>[2x]MAAQGPSPIPTNRLKQIAADACNDAIGSAEFYDHAKTEQWNHQIINTILKAVIAESQPSDSTTPPQFKFAVNSTIVQHLVPSSKLNKPAGGADDKPASTATSTDGKPHVGRRG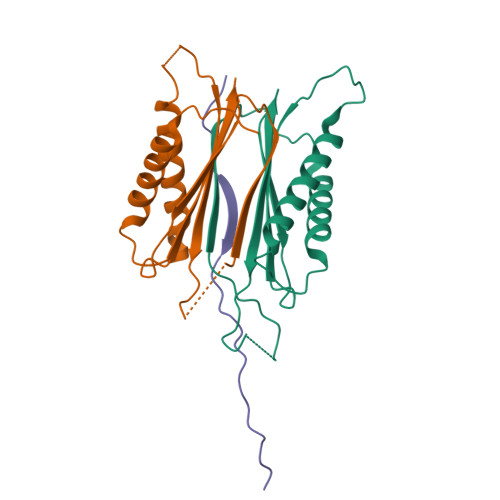MHSATGAFWNDKTDGMWTYKHEGDESKGMDVVVMLIWIAVLEHHHHHH;> AAPQNLTTVPLTTIYECPPSPVKEIFSYSKGIQTQ>[2x]MATKSDGSASAAAEGGARKTNIEAYRDGLKLKTEEDFFACDRQYVCQNYAPVPVVISKGKGARVWDINGNEY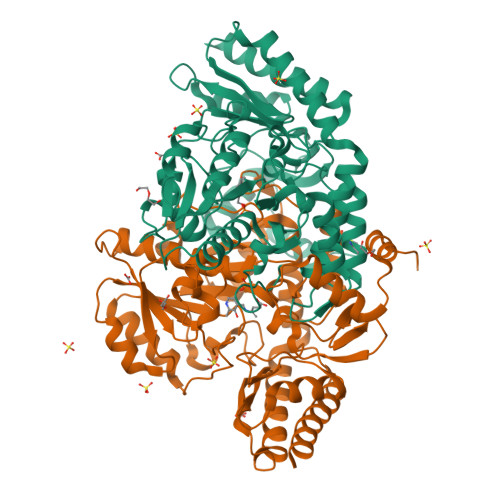YDFLAGVSSLSQGHCHPRVIAALCRQAERLTLTLRAFGNDVTGPACRFMAEMFGYDRVLLMNTGAEAGESALKIARKWAYEVKEIPPDSAKVILCNNNYWGRTITACSSSTTFDCYNNFGPFTPGFELIDYDDVGALEEALKDPNVAAFFVEPIQGEGGVNVPKPGYLKRAHELCRSKNVLLIVDEIQTGLCRTGRLLAADHDEVHPDILLLGKSLSAGVVPISAVMGRADVMDVLKPGTHGSTFGGNPLACAVAVEALTVLKDEKLADRAERLGAQFRDCLRRELYGKVPWIKEIRGRGLLNAVEVDSDAIDPNDVVMKLKENGILSKPTRGRVMRFIPPLVITDEEHRDATTRIIKSFLAVEEERKK>[2x]MFRKLAAECFGTFWLVFGGCGSAVLAAGFPELGIGFAGVALAFGLTVLTMAFAVG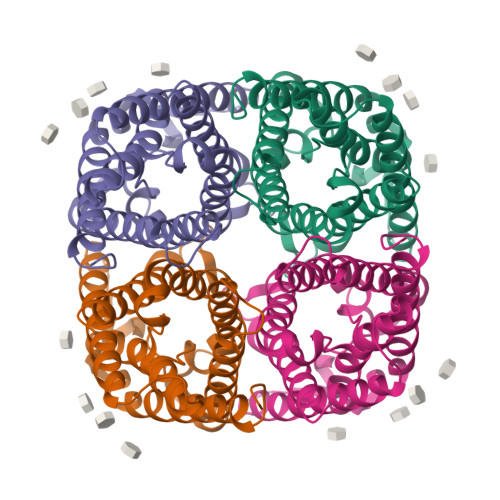HISGGHFNPAVTIGLWAGGRFPAKEVVGYVIAQVVGGIVAAALLYLIASGKTGFDAAASGFASNGYGEHSPGGYSMLSALVVELVLSAGFLLVIHGATDKFAPAGFAPIAIGLALTLIHLISIPVTNTSVNPARSTAVAIFQGGWALEQLWFFWVVPIVGGIIGGLIYRTLLEKRD>MARRLPKPTLQGRLEADFPDSPLLPKFQELNQNNLPNDVFREAQRSYLVFLTSQFCYEEYVQRTFGVPRRQRAIDKRQRASVAGAGAHAHLGGSSATPVQQAQAAASAGTGALASSAPSTAVAQSATPSVSSSISSLRAATSGATAAASAAAAVDTGSGGGGQPHDTAPRGARKKQ[5x];>MKVQGSVDRRRLQRRIAGLLPPPARRLNISRGSEFTRDVRGLVEEHAQASSLSAAAVWRAGLLAPGEVAVAGGGSGGGSFSWSGWRPPVFGDFLIHASSFNNAEATGTPLFQFKQSDPFSGVDAVFTPLSLFILMNHGRGVAARVEAGGGLTRMANLLYDSPATLADLVPDFGRLVADRRFHNFITPVGPLVENIKSTYLNKITTVVHGPVVSKAIPRSTVKVTVPQEAFVDLDAWLSGGAGGGGGVCFVGGLGLQPCPADARLYVALTYEEAGPRFTFFQSSRGHCQIMNILRIYYSPSIMHRYAVVQPLHIEELTFGAVACLGTFSATDGWRRSAFNYRGSSLPVVEIDSFYSNVSDWEVIL[2x];>MDLKVVVSLSSRLYTDEIAKMQQRIGCILPLASTHGTQNVQGLGLGQVYSLETVPDYVSMYNYLSDCTLAVLDEVSVDSLILTKIVPGQTYAIKNKYQPFFQWHGTGSLSVMPPVFGREHATVKLESNDVDIVFPMVLPTPIAEEVLQKILLFNVYSRVVMQAPGNADMLDVHMHLGSVSYLGHHYELALPEVPGPLGLALLDNLSLYFCIMVTLLPRASMRLVRGLIRHEHHDLLNLFQEMVPDEIARIDLDDLSVADDLSRMRVMMTYLQSLASLFNLGPRLATAAYSQETLTATCWLR[4x];>MSNGDWGQSQRTRGTGPVRGIRTMDVNAPGGGSGGSALRILGTASCNQAHCKFGRFAGIQCVSNCVLYLVKSFLAGRPLTSRPELDEVLDEGARLDALMRQSGILKGHEMAQLTDVPSSVVLRGGGRVHIYRSAEIFGLVLFPAQIANSAVVQSLAEVLHGSYNGVAQFILYICDIYAGAIIIETDGSFYLFDPHCQKDAAPGTPAHVRVSTYAHDILQYVGAPGAQYTCVHLYFLPEAFETEDPRIFMLEHYGVYDFYEANGSGFDLVGPELVSSDGEAAGTPGADSSPPVMLPFERRIIPYNLRPLPSRSFTSDSFPAARYSPAKTNSPPSSPASAAPASAAPASAAPASAAPASAAPASAAPASAAPASAAPASSPPLFIPIPGLGHTPGVPAPSTPPRASSGAAPQTPKRKKGLGKDSPHKKPTSGRRLPLSSTTDTEDDQLPRTHVPPHRPPSAARLPPPVIPIPHQSPPASPTPHPAPVSTIAPSVTPSPRLPLQIPIPLPQAAPSNPKIPLTTPSPSPTAAAAPTTTTLSPPPTQQQPPQSAAPAPSPLLPQQQPTPSAAPAPSPLLPQQQPPPSAARAPSPLPPQQQPLPSATPAPPPAQQLPPSATTLEPEKNHPPAADRAGTEISPSPPFGQQPSFGDDASGGSGLVRYLSDLEEPFLSMSDSEEAESDLASDIPTTEDEDMFEDEVFSNSLESGSSAPTSPITLDTARSQYYQTTFDIETPEMDFVPLESNIARIAGHTYQEQAIVYDPASNREVPEADALSMIDYLLVTVVLEQGLIRSRDRSSVLNLLEFLKDWSGHLQVPTLDLEQLLTSELNIQNLANMLSENKGRAGEFHKHLAAKLEACLPSLATKDAVRVDAGAKMLAEIPQLAESDDGKFDLEAARRRLTDLLSGGDQEAGEGGGEPEDNSIYRGPHVDVPLVLDDESWKRLLSLAEAARTAVARQQAGVDEEDVRFLALLTAIEYGAPPAASVPPFVHNVAVRSKNAALHVRRCTADIRDKVASAASDYLSYLEDPSLPTVMDFDDLLTHLRHTCQIIASLPLLNIRYTSIEWDYRELLYLGTALSDMSGIPWPLERVEEDDPSIAPLPEFETVAKKQKELETTRENEKRLRTILDDIEAMLGLAGVASAPGAPISPASPSATPANHDNPEATPPLADTAALTIPVIEKYIANAGSIVGAAKNPTYIRLRDTIQQIVRSKKYLMNILKSITFYTIDNYIASFEESIDHLYRDLPVLDPEVQDGIDRILDPMVSEALHTFEMGNRLTLEPARLVALQNFATHSTLKETAAAVNLLPGLLAVYDATITGQAPEDALRLLSGLQNQLSQTLIPGKLKKRFLSYLQKLKNNNNDQLRQKEVQAWRLEAEGFKPATEEQLEAFLDTAPNKELKRQYEKKLRQLMETGRKEKEKLREQEDKERQERRAREANEAWARIRKALGARPEPAPTSPDDWNTLLASLLPDNTDSAAAAAAAVARNTDILDSLTQILAAMLLGITRVRRERLRSLLVDDGGAAERMEAAEPGWFTDIETGPLARLDAWPATPAATAKEGGGGRGAEEAAGALFRARTAADAIRSALAQTRQALQSPDMKSAVVNTDLEAPYAEYERGLAGLLEKRRAAEAALTAIVSEYVDRTLPEATNDPGQANLPPPPTIPQATAPPRLASDSALWPKKPQLLTRRERDDLLQATGDFFSELLTEAEAAEVRALEEQVRESQTLMAKAHEMAASTRRGFHTALEAVLSRSRDEAPDDELRSLLPSPPKAPVQAPLEAALARAAAGNGSWPYRKSLAAAKWIRGICEAVRGLSEGALALAGGAGAWLNLAAAADGEIHELTRLLEVEGMAQNSMDGMEELRLALATLDPKRVAGGKETVADWKRRLSRLEAIIQEAQEESQLQGTLQDLVTQARGHTDPRQLKIVVEAARGLALGASAGSQYALLKDKLLRYASAKQSFLAFYETAQPTVFVKHPLTNNLPLLITISAPPTGWGNGAPTRRAQFLAAAGPAKYAGTLWLETESPCDPLNPAYVSADTQEPLNYIPVYHNFLEYVMPTVLENPEAFSLTPAGRPQAIGPPQDDQERRRRTLASVASARLSAAAADSYWDTWPDVESNAGELLREYVSAPKALMEDLADNPIVAMTLLAHASLIASRNHPPYPAPATDREVILLEQREMMALLVGTHPAYAAAFLGAPSFYAGLGLVSALARDGGLGDLLSDSVLTYRLVRSPASGRGGMPSTTRGSNDGEDARRLTRHRIAGPPTGFIFFQDAWEEMDTRAALWPHPEFLGLVHNQSTARARACMLLLARRCFAPEALQQLWHSLRPLEGPVAFQDYLRDFVKQAYTRGEELPRAEGLEVPRETPSSYGTVTGRALRNLMPYGTPITGPKRGSGDTIPVSVFEAAVAAAFLGRPLTLFVSSQYLFNLKTLGQVRVVAPLLYCDGHSEPFRSLVETISLNFLQDLDGYSESFEPEMSIFARQAVWLRELLTEARAAKPKEARPPTVAILANRKNIIWKCFTYRHNLPDVQFYFNAAGASRWPTDVLNPSFYEHEDPPLPVGYQLPPNPRNVQELFSGFPPRVGHGLVSGDGFQSADNTPASSDRLQQLGGGETDQGEKGSTTAESEASGPPSPQSPLLEKVAPGRPRDWLSPTSSPRDVTVTPGLAAPITLPGPRLMARPYFGAETRASESPDRSPGSSPRPWPKDSLELLPQPAPQQPPSSPWASEQGPIVYTLSPHSTPSTASGSQKKHTIQIPGLVPSQKPSYPPSAPYKPGQSTGGIAPTPSAASLTTFGLQPQDTQASSQDPPYGHSIMQREKKQQGGREEAAEIRPSATRLPTAVGLRPRAPVVAAGAAASATPAFDPGEAPSGFPIPQAPALGSGLAAPAHTPVGALAPRPQKTQAQRPQDAAALPTPTIKAVGARPVPKATGALAAGARPRGQPTAAPPSAASPPRVSLPVRSRQQQSPAIPLPPMHSGSEPGARPEVRLSQYRHAGPQTYTVRKEAPPSAASQLPKMPKCKDSMYYPPSGSARYPAPFQALSFSQSVASPAPSSDQTTLLWNTPSVVTQFLSIEDIIREVVTGGSTSGDLVVPSGSPSSLSTAAPEQDLRYSLTLSQASRVLSRFVSQLRRKLERSTHRLIADLERLKFLYL[2x];> MDVHIDNQVLSGLGTPLLVHLFVPDTVMAELCPNRVPNCEGAWCQTLFSDRTGLTRVCRVFAARGMLPGRPSHRGTFTSVPVYCDEGLPELYNPFHVAALRFYDEGGLVGELQIYYLSLFEGAKRALTDGHLIREASGVQESAAAMQPIPIDPGPPGGAGIEHMPVAAAQVEHPKTYDLKQILLEITQEENRGEQRLGHAGSPALCLGLRLRAGAETKAAAETSVSKHHPALENPSNIRGSAGGEGGGGRAGTGGTVGVGSGALSRVPVSFSKTRRAIRESRALVRGIAHIFSPHALYVVTYPELSAQGRLHRMTAVTHASPATDLAEVSILGAPEREFRFLISVALRISASFREKLAMQAWTAQQEIPVVIPTSYSRIYKNSDLIREAFFTVQTRVSWESCWVKATISNAPKTPDACLWIDSHPLYEEGASAWGKVIDSRPPGGLVGAASQLVALGTDGHCVHLATTSDGQAFLVLPGGFVIKGQLALTPEERGYILARHGIRREQ;>[2x]MALSGHVLIDPARLPRDTGPELMWAPSLRNSLRVSPEALELAEREAERARSERWDRCAQVLKNRLLRVELDGIMRDHLARAEEIRQDLDAVVAFSDGLESMQVRSPSTGGRSAPAPPSPSPAQPFTRLTGNAQYAVSISPTDPPLMVAGSLAQTLLGNLYGNINQWVPSFGPWYRTMSANAMQRRVFPKQLRGNLNFTNSVSLKLMTEVVAVLEGTTQDFFSDVRHLPDL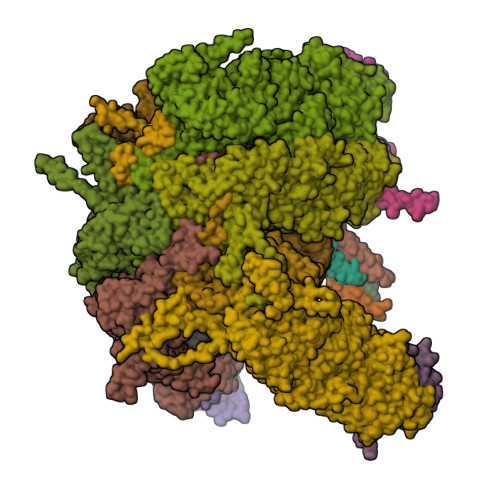QAALILSVAYLLLQGGSSHQQRPLPASREELLELGPESLEKIIADLKAKSPGGNFMILTSGNKEARQSIAPLNRQAAYPPGTFADNKIYNLFVGAGLLPTTAALNVPGAAGRDRDLVYRIANQIFGEDVPPFSSHQWNLRVGLAALEALMLVYTLCETANLAEAATRRLHLSSLLPQAMQRRKPAMASAGMPGAYPVQTLFRHGELFRFIWAHYVRPTVAADPQASISSLFPGLVLLALELKLMDGQAPSHYAINLTGQKFDTLFEIINQKLLFHDPAAMLAARTQLRLAFEDGVGVALGRPSPMLAAREILERQFSASDDYDRLYFLTLGYLASPVAPS;>[5x]MASNEGVENRPFPYLTVDADLLSNLRQSAAEGLFHSFDLLVGKDAREAGIKFEVLLGVYTNAIQYVRFLETALAVSCVNTEFKDLSRMTDGKIQFRISVPTIAHGDGRRPSKQRTFIVVKNCHKHHISTEMELSMLDLEILHSIPETPVEYAEYVGAVKTVASALQFGVDALERGLINTVLSVKLRHAPPMFILQTLADPTFTERGFSKTVKSDLIAMFKRHLLEHSFFLDRAENMGSGFSQYVRSRLSEMVAAVSGESVLKGVSTYTTAKGGEPVGGVFIVTDNVLRQLLTFLGEEADNQIMGPSSYASFVVRGENLVTAVSYGRVMRTFEHFMARIVDSPEKAGSTKSDLPAVAAGVEDQPRVPISAAVIKLGNHAVAVESLQKMYNDTQSPYPLNRRMQYSYYFPVGLFMPNPKYTTSAAIKMLDNPTQQLPVEAWIVNKNNLLLAFNLQNALKVLCHPRLHTPAHTLNSLNAAPAPRDRRETYSLQHRRPNHMNVLVIVDEFYDNKYAAPVTDIALKCGLPTEDFLHPSNYDLLRLELHPLYDIYIGRDAGERARHRAVHRLMVGNLPTPLAPAAFQEARGQQFETATSLAHVVDQAVIETVQDTAYDTAYPAFFYVVEAMIHGFEEKFVMNVPLVSLCINTYWERSGRLAFVNSFSMIKFICRHLGNNAISKEAYSMYRKIYGELIALEQALMRLAGSDVVGDESVGQYVCALLDPNLLPPVAYTDIFTHLLTVSDRAPQIIIGNEVYADTLAAPQFIERVGNMDEMAAQFVALYGYRVNGDHDHDFRLHLGPYVDEGHADVLEKIFYYVFLPTCTNAHMCGLGVDFQHVAQTLAYNGPAFSHHFTRDEDILDNLENGTLRDLLEISDLRPTVGMIRDLSASFMTCPTFTRAVRVSVDNDVTQQLAPNPADKRTEQTVLVNGLVAFAFSERTRAVTQCLFHAIPFHMFYGDPRVAATMHQDVATFVMRNPQQRAVEAFNRPEQLFAEYREWHRSPMGKYAAECLPSLVSISGMTAMHIKMSPMAYIAQAKLKIHPGVAMTVVRTDEILSENILFSSRASTSMFIGTPNVSRREARVDAVTFEVHHEMASIDTGLSYSSTMTPARVAAITTDMGIHTQDFFSVFPAEAFGNQQVNDYIKAKVGAQRNGTLLRDPRTYLAGMTNVNGAPGLCHGQQATCEIIVTPVTADVAYFQKSNSPRGRAACVVSCENYNQEVAEGLIYDHSRPDAAYEYRSTVNPWASQLGSLGDIMYNSSYRQTAVPGLYSPCRAFFNKEELLRNNRGLYNMVNEYSQRLGGHPATSNTEVQFVVIAGTDVFLEQPCSFLQEAFPALSASSRALIDEFMSVKQTHAPIHYGHYIIEEVAPVRRILKFGNKVVF> MSNEDYGYDYDY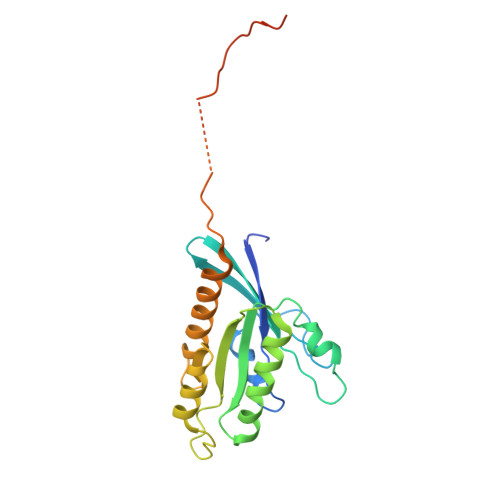LFKIVLIGDSGVGKSNLLSRFTTDEFNIESKSTIGVEFATRTIEVENKKIKAQIWDTAGQERYRAITSAYYRGAVGALIVYDISKSSSYENCNHWLTELRENADDNVAVGLIGNKSDLAHLRAVPTDEAKNFAMENQMLFTETSALNSDNVDKAFRELIVAIFQMVSKHQVDLSGSGTNNMGSNGAPKGPTISLTPAPKEDKKKKSSNHHHHHHH In the present study, we characterized a GH146 β-l-arabinofuranosidase, Bll3HypBA1 (BLLJ_1848), which was found to constitute a gene cluster with AGP-degrading enzymes. Bll3HypBA1 also exhibited < 1% degradative activity for Araf-β-pNP, Araf-β-OMe, Araf-β-Hyp glycosides, and β-AOSs containing Araf-β1,2-linkage compared with Araf-β1,3-ArafGal2 containing Araf-β1,3-linkage. These results showed that Bll3HypBA1 is a β-l-arabinofuranosidase specific for Araf-β1,3-Araf structures. The crystal structure of GH146 Bll3HypBA1 consists of three domains: catalytic (α/α)6 barrel (aa: 379–820), β-sandwich 1 (aa: 821–920), and β-sandwich 2 (aa: 921–1051). The Zn atom of Bll3HypBA1 is coordinated by Cys3-Glu residues, and GH127 and GH146 enzymes share this structural characteristic.

To obtain a clone suitable for X-ray crystallography and biochemical analysis, we constructed Bll3HypBA1-NΔ379CΔ761 and Bll3HypBA1-NΔ379CΔ933 without the LamG region. The crystal structure of Bll3HypBA1-NΔ379CΔ761 (aa: 380–1223) was determined at a resolution of 1.75 Å by the single-wavelength anomalous dispersion using a SeMet-derivative. The NΔ379CΔ761 structure contained one molecule per asymmetric unit, and residues M379–V1051 were modeled. In the active site of the NΔ379CΔ761 structure, a Zn atom coordinated by E723, C725, C804, and C805 was clearly observed, and a Tris molecule was bound to the l-arabinose-binding site (subsite − 1). A crystallographic anomalous scattering analysis was performed to identify the metal atom. A Bijvoet difference density map of the data collected at 1.280 Å wavelength revealed a prominent peak at the metal site, whereas a difference map of the data collected at 1.300 Å wavelength, which is above the absorption edge of Zn (1.2837 Å), showed a significant decrease in the anomalous scattering ability. This result confirmed that the metal ion bound at the active site is Zn2+. The three molecules, including one in NΔ379CΔ761 and two in NΔ379CΔ933, had almost identical main chain structures, as the root mean square deviation (RMSD) values for the Cα atoms between all chain pairs were less than 0.24 Å. The estimated molecular masses by gel filtration chromatography were 91 kDa and 76 kDa for Bll3HypBA1-NΔ379CΔ761 and Bll3HypBA1-NΔ379CΔ933, respectively, suggesting that both protein constructs are monomeric in solution (data not shown).

> MENVTVADEYLQNAGKKEVEYLLSFEPDRLLVEFRAQAGLDTKGAKNYGGWENGPDESRNPDGSSKPGRFTGHFVGHWISAASQAQRSTFATADQKAQLSANLTAVVKGIREAQEAYAKKDTANAGFFPAFSASVVPNGGGGLIVPFYNLHKVEAGMVQAYDYSTDAETRETAKAAAVDFAKWVVNWKSAHASTDMLRTEYGGMNDALYQVAEIADASDKQTVLTAAHLFDETALFQKLANGQDPLNGLHANTTIPKLTGAMQRYVAYTEDEDLYNSLSADERGKLTSLYLKAAQNFFDIVVKDHTYVNGGNSQSEHFHVAGELWKDATQNGDQNGGYRNFSTVETCNEYNMLKLARILFQVTKDSKYSEYYEHTFINAIVASQNPETGMTTYFQPMKAGYPKVFGITGTDYDADWFGGAIGEYWCCQGTGIENFAKLNDSFYFTDENNVYVNMFWSSTYTDTRHNLTITQTANVPKTEDVTFEVSGTGSANLKLRVPDWAITNGVKLVVDGTEQALTKDENGWVTVAIKDGAKITYTLPAKLQAIDAADNKDWVAFQYGPVVLAGALTDTNYKTNYSYGGVKVRVANYDSEANAKAAVIPTSGSVTDWLKGIKEDASEGSNLVRTDDPNTGNRETLSFKFANVDGDAADLTLQPYYSTYKTTYAIYWDMAEVDSETYQNNIFKKKTDAATQSIIIDAVDAFDNEFQQELAHNAAKSDDSNAGTYEDKQYRDAKADGWFSYDLKVNTEADAKNYLSVQYQSADAGRTFSMIVDPTPVADNSKGEVSANAKTYTVTIENKGLKAFYWDVQQLPADLIAEAKDGKVRVLFKSTGGLVGGVYGVRMQNAAALEHHHHHH> AMPVFHTRTIESILEPVAQQISHLVIMHEEGEVDGKAIPDLTAPVSAVQAAVSNLVRVGKETVQTTEDQILKRDMPPAFIKVENACTKLVRAAQMLQADPYSVPARDYLIDGSRGILSGTSDLLLTFDEAEVRKIIRVCKGILEYLTVAE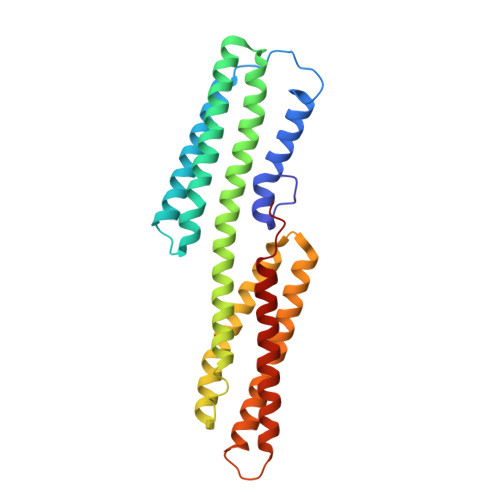VVETMEDLVTYTKNLGPGMTKMAKMIDERQQELTHQEHRVMLVNSMNTVKELLPVLISAMKIFVTTKNTKSQGIEEALKNRNFTVEKMSAEINEIIRVLQLTSWD>[2x]SNAGAPLKAVSAFAPPMKTQDFNLYTNEVHAKFDDYDLGMEYARQHNKPVMLDFTGYGCVNCRKMELAVWTDPKVSSIINNDYVLITLYVDNKTPLTEPVKIME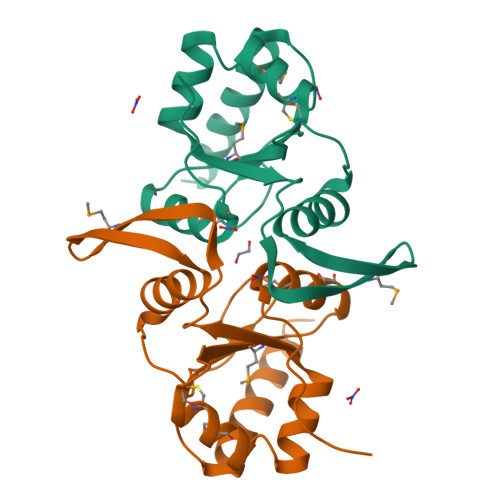NGTERTLRTVGDKWSYLQRVKFGANAQPFYVLIDNEGNPLNKSYAYDEDISKYINFLQTGLENYRKEK> GSMSKKPTAGPALHKVIMVGSGGVGKSALTLQFMYDEFVEDYEPTKADSYRKKVVLDGEEVQIDILDTAGQEDYAAIRDNYFRSGEGFLCVF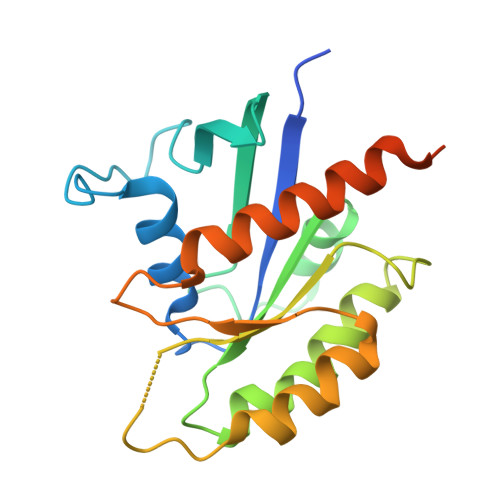SITDDESFQATQEFREQILRVKNDESIPFLLVGNKCDLNDKRKVPLSECQLRAQQWAVPYVETSAKTRENVDKVFFDLMREIRSRKTEDSKATSGRAKDRCKKRRLKCTLL>LKNANLDPKTRVLEHRLLAASSAIAEKLGVSAGDEVLLIRRLRSTGDIPVAILENYLPPAFNDVSLDELEKGGLYDALRSRGVVLKIANQKIGARRAVGEESTLLDIEDGGPLLTVERVALDNSGQVIELGSHC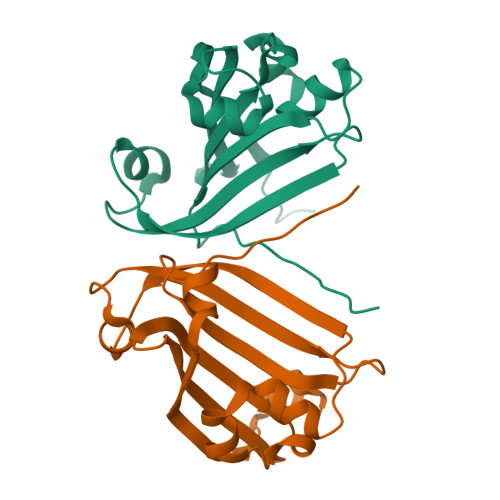YRPDMYNFETTLVAR[3x]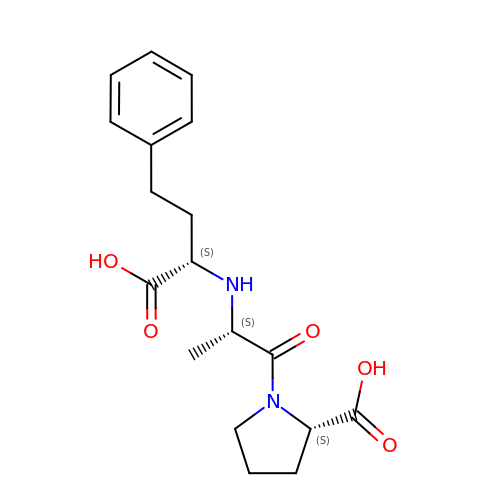1-((2S)-2-{[(1S)-1-CARBOXY-3-PHENYLPROPYL]AMINO}PROPANOYL)-L-PROLINE | C18 H24 N2 O5 | LZFZMUMEGBBDTC-QEJZJMRPSA-N>MHHHHHHHHMDSRSPSLPDDRPDPPEQHLDARAGATLRGTAGPRGVRRILPFLRPAVIASIAYMDPGNFATNIEGGARYGYSLLWVILAANLMAMVIQNLSANLGIASGRNLPELIRERWPRPLVWFYWIQAELVAMATDLAEFLGAALAIQLLTGLPMFWGAVVTGVVTFWLLNLQKRGTRPLELAVGAFVLMIGVAYLVQVVLARPDLAAVGAGFVPRLQGPGSAYLAVGIIGATVMPHVIYLHSALTQGRIQTDT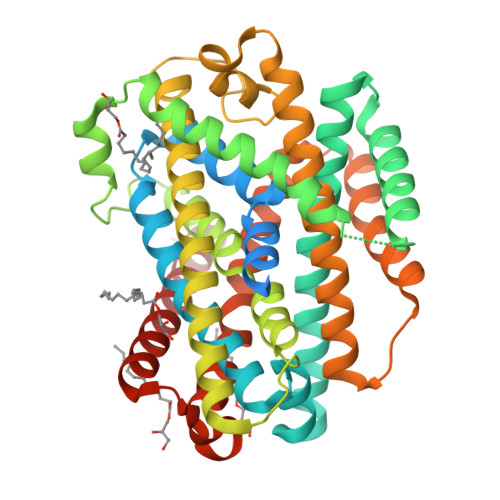TEEKRRLVRLNRVDVIAAMGLAGLINMSMLAVAAATFHGKNVENAGDLTTAYQTLTPLLGPAASVLFAVALLASGLSSSAVGTMAGDVIMQGFMGFHIPLWLRRLITMLPAFIVILLGMDPSSVLILSQVILCFGVPFALVPLLLFTARRDVMGALVTRRSFTVIGWVIAVIIIALNGYLLWELLGG[2x]> MTYNELIYMVLDELKLSSDDSYYTPDHVIFLLVKYRSFLLKQRYSDIK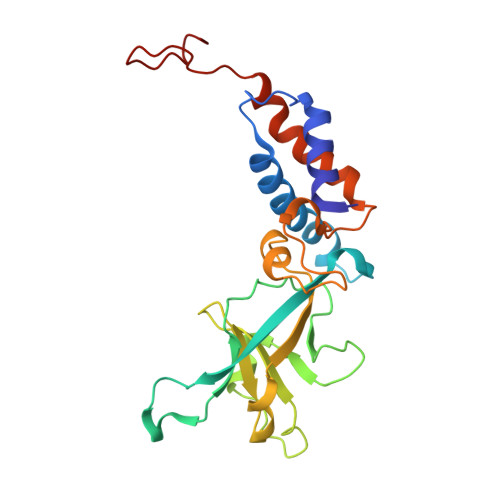KQIPDSDYQSICLDLIEVPAISGEPCEGSSYLRSKNKVPTTMMIGNPRVYPMDFYQGEITYISRDRMRYVGYNKFLRNIIYCSKAPDGYLYFKSWNPQFLHLEKVSFNAIFEDAKEASEMACPEENGTICKLEDKEFPIEDALVPPLIELVVKELRGPEYSPKDEDNNAKDDLPDAR> MAESFFSDFGLLWYLKELRKEEFWKFKELLKQPLEKFELKPIPWAELKKASKE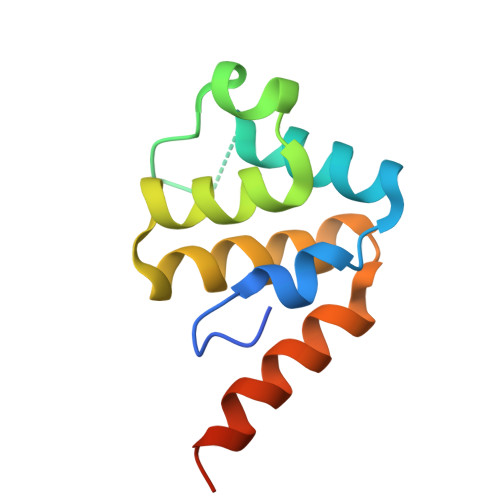DVAKLLDKHYPGKQAWEVTLNLFLQINRKDLWTKAQEEMRNKLLEHHHHHH>MNVPDMILYNGKITTLDPSQPEVSAIAITDGLITAVGGDELLNSATEKTKKIDLKRKRAIPGLNDSH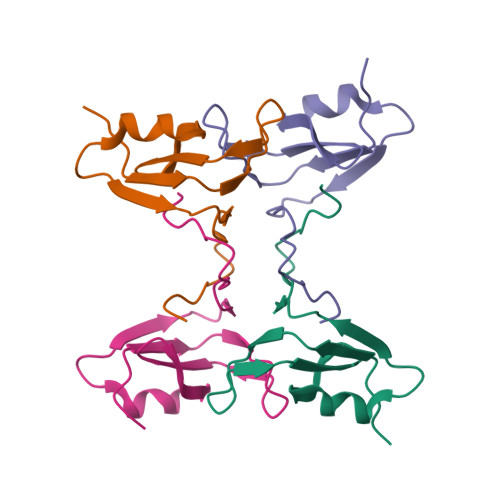IHVIRGLEHHHHHH[4x]>MD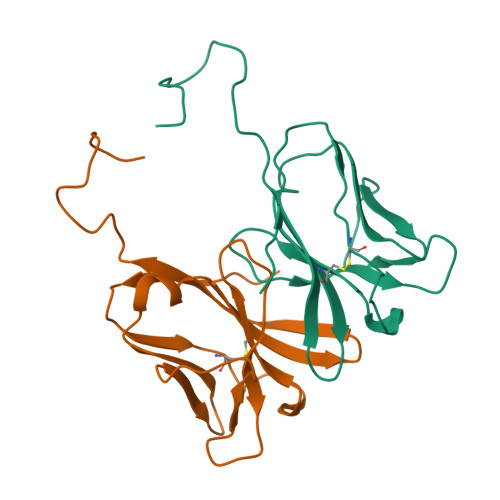IKELHVKTVKRGENVTMECSMSKVTNKNNLAWYRQSFGKVPQYFVRYYSSNSGYKFAEGFKDSRFSMTVNDQKFDLNIIGAREDDGGEYFCGEVEGIIIKFTSGTRLQFEGSNEGSKSSDGEGSSCPDQMHVLVW[6x]4-cyano-N-[(1S,2R)-2-phenylcyclopropyl]benzamide | C17 H14 N2 O | 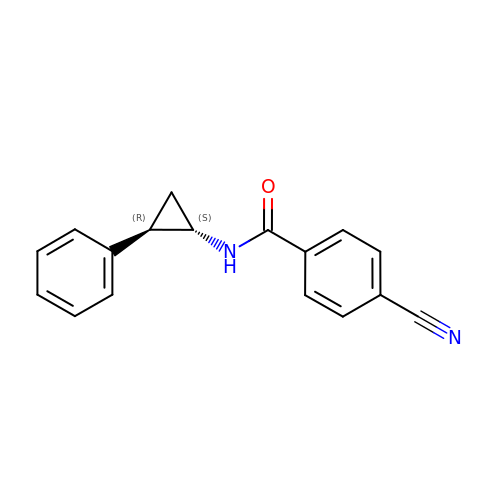RPFFDFASGIBGIP-CVEARBPZSA-N>GAMAFEDRDPTQFEERHLKFLQQLGKGNFGSVEMCRYDPLQDNTGEVVAVKKLQHSTEEHLRDFEREIEILKSLQHDNIVKYKGVCYSAGRRNLKLIMEYLPYGSLRDYLQKHKERIDHIKLLQYTSQICKGMEYLGTKRYIH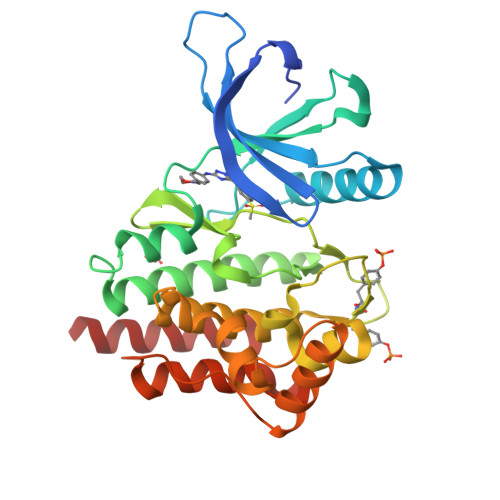RDLATRNILVENENRVKIGDFGLTKVLPQDKEYYKVKEPGESPIFWYAPESLTESKFSVASDVWSFGVVLYELFTYIEKSKSPPAEFMRMIGNDKQGQMIVFHLIELLKNNGRLPRPDGCPDEIYMIMTECWNNNVNQRPSFRDLALRVDQIRDNMAG[2x]> MAGLPEARKLLGLAYPERRRLAAAVGFLTMSSVISMSAPFFLGKIIDVIYTNPTVDYSDNLTRLCLGLSAVF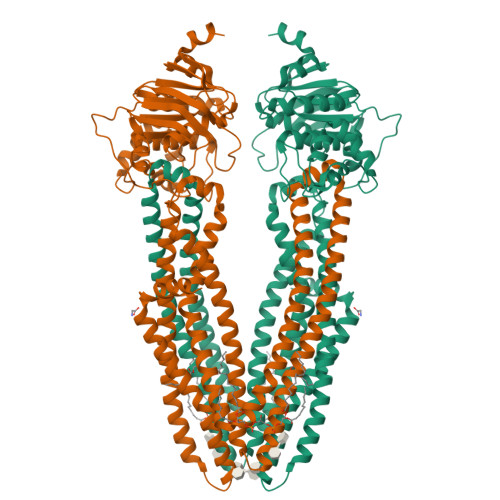LCGAAANAIRVYLMQTSGQRIVNRLRTSLFSSILRQEVAFFDKTRTGELINRLSSDTALLGRSVTENLSDGLRAGAQASVGISMMFFVSPNLATFVLSVVPPVSIIAVIYGRYLRKLTKVTQDSLAQATQLAEERIGNVRTVRAFGKEMTEIEKYASKVDHVMQLARKEAFARAGFFGATGLSGNLIVLSVLYKGGLLMGSAHMTVGELSSFLMYAFWVGISIGGLSSFYSELMKGLGAGGRLWELLEREPKLPFNEGVILNEKSFQGALEFKNVHFAYPARPEVPIFQDFSLSIPSGSVTALVGPSGSGKSTVLSLLLRLYDPASGTISLDGHDIRQLNPVWLRSKIGTVSQEPILFSCSIAENIAYGADDPSSVTAEEIQRVAEVANAVAFIRNFPQGFNTVVGEKGVLLSGGQKQRIAIARALLKNPKILLLDEATSALDAENEYLVQEALDRLMDGRTVLVIAHRLSTIKNANMVAVLDQGKITEYGKHEELLSKPNGIYRKLMNKQSFISAAENLYFQ>GHMERLLDELTLEGVARYMQSERCRRVICLVGAGISTSAGIPDFRSPSTGLYDNLEKYHLPYPEAIFEISYFKKHPEPFFALAKELYPGQFKPTICHYFMRLLKDKGLLLRCYTQNIDTLERIAGLEQEDLVEAHGTFYTSHCVSASCRHEYPLSWMKEKIFSEVTPKCEDCQSLVKPDIVFFGESLPARFFSCMQSDFLKVDLLLVMGTSLQ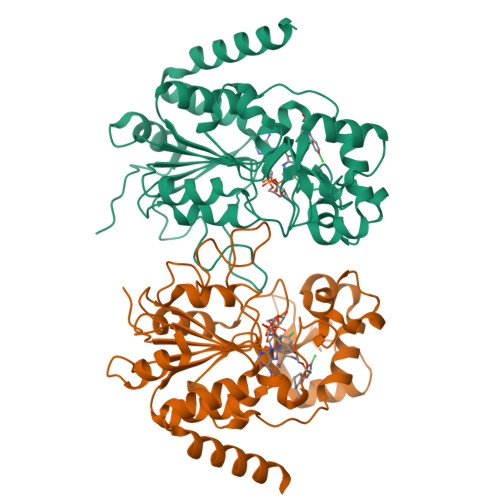VQPFASLISKAPLSTPRLLINKEKAGQSDPFLGMIMGLGGGMDFDSKKAYRDVAWLGECDQGCLALAELLGWKKELEDLVRREHASIDAQS[2x]>MKKDLKFIKSVYDLKSFSDKAAFAKKTFKDEGGIILARNLEHVSSEIFTQEFAGLTFLQGGIVVNNEGGYATSVTKLKLKAEGGFRESGNDTNTTGKITLSGESDSIPVFTLEGESDWSEIELKQAELQNVNLPSRYFEAHAELYNRKIDELGYLGQTRTDGTQKTLGLLNYGFVASGAGDTAANLSGDNLYQAIADLITDQWAGVFNVETYKADRVVMPDTVYNICAKKILNSNGSEMSVLRALMTNFPTVTFGLTTKARDVGGTSRTTAYSSNRRAMQMRIPTPLNVSSVDQRGFKYYVESYFGVAGLDVIEDTAGRHLTGL[7x];>[7x]MAFNNAVLQEVSDLPAGEVIKASPHNVSAFEVFQNGLIEGRFVKFDAGSIDILDASATPTIAGIAKRKVT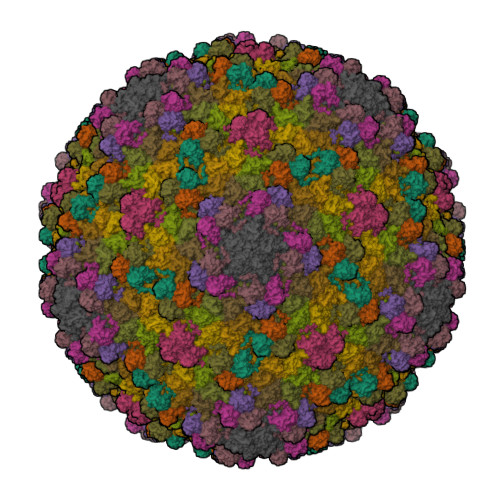GEIGPGVYSTSGIEIDQVAEVINFGFATVTVQDAAAPSKYDPVYAINLDSAEAGKATENSGATGALAVADCVFWEQKAANVWLVRMNKFL>EIVTDNSTGNHDGYDYEFWKDSGGSGTMILNSGGTFSASWSSVSNILFRKGKKFNETQTHQQVGNMSISYGANFQPSGNAYLCVYGWTVSPLVEYYIVDSWGNWRPPGATPKGTITVDGGTYDIYET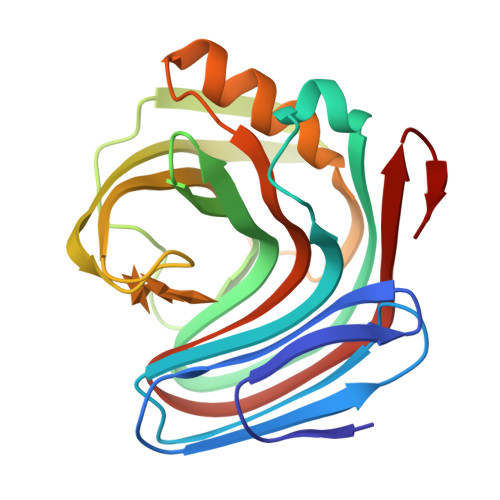DRTNQPSIKGVATFSQYWSTRRSKRTSGTISVSNHFRAWESLGMNMGDMYEVALTVEGYQSSGSANVYSNTLRINGNPL[2x]5-(methylsulfanyl)-4-(propan-2-ylsulfonyl)-1H-pyrazol-3-amine | C7 H13 N3 O2 S2 | 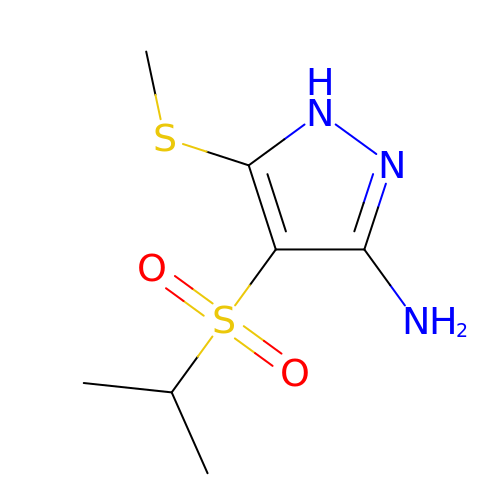SEBINQGTUBTFET-UHFFFAOYSA-N>MVSKADNSAKLVEGKAKPMGSFPHVKRAGDFLFVSGTSSRRPDNTFVGAEPDDTGRPRPNIELQTREVISNIRDILQSVGADLGDVVEVCSYLVNMNDFAAYNKVYAEFFDATGPARTTVAVHQLPHPQLVIEIKVVAYKPL[9x]

The amnE gene product AmnE is a deaminase, and hydrolyzes 2-aminomuconate to 4-oxalocrotonate and releases ammonia in the modified meta-cleavage pathway. The deduced amino acid sequence of 2-aminomuconate deaminase in Pseudomonas sp. AP–3 shows that AmnE belongs to a member of the YjgF/YER057c/UK114 protein family. The metabolic pathway for 2-aminophenol in Pseudomonas sp. AP–3 is referred to as the modified meta-cleavage pathway, in which 2-aminomuconate is transformed into 4-oxalocrotonate by the deaminase AmnE. In this study, we demonstrate that AmnE self-assembles in a unique homo-hexameric form that is different from a regular trimer model of the RidA subfamily.

The homohexameric structure of AmnE has been determined at a high resolution (equal to 1.75 Å), and constitutes the first protein structure in the metabolic pathway of 2-aminophenol. The crystal structure of AmnE was solved in the space group C121 with nine protomers (A, B, C, D, E, F, G, H, I) composed of three identical homotrimers (trimers I, II, and III) in one asymmetric unit. One of the AmnE hexamers is organized based on the use of two identical trimers, trimer I (A/B/C) and trimer II (D/E/F). Trimer III forms a hexamer with the use of trimer III in the neighboring asymmetric unit in the crystal lattice. The overall structure of the AmnE protomer shows an α + β fold with a β-sheet (β1 - β6), two α-helices (α1, α4), and two 310-helices (α2, α3), in an arrangement of β1 (residues 9 –10), β2 (residues 25–28), β3 (residues 31–37), α1 (residues 61 –78), α2 (residues 83–85), β4 (residues 86–93), β3 (residues 96–98), α4 (residues 99–106), β5 (residues 116–121), and β6 (residues 132–139). Lp2 (residues 38–60) is the longest loop and connects β3 and α1. In the AmnE hexameric structure, two trimers (trimer I, timer II) interact in a back-to-back manner through the hydrophobic region composed of six Lp3 loops (Lp3A, Lp3B, and Lp3C, from trimer I, and Lp3D, Lp3E, Lp3F, from trimer II). Six residues His123 (His123A–F), located on the loops Lp3, form a hydrophobic base with residues Val122A–F, Leu125A–F, and Leu130A–F present in the AmnE hexamer. Outside of the hexamer, six loops (Lp2A, Lp2B, and Lp2C, from trimer I, and Lp2D, Lp2E, and Lp2F, from trimer II) surround the hexamer and extend into the cleft area of the opposite trimer to form a solid football-like shape. There are six pivotal residues Arg56 (Arg56A–F) located on loops Lp2 (Lp2A–F) that formed eighteen hydrogen bonds in the hexamer with residues Pro126 (Pro126A–F) and Met96 (Met96A–F).> 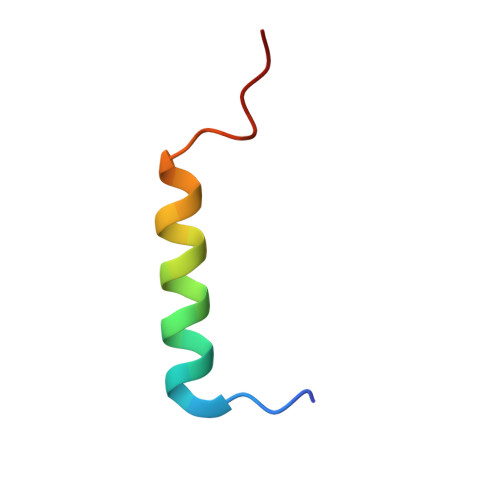HMWETLDDQRALQLALDQLSLLGLDSDE> MARKQNRNSKELGLVPLTDDTSHAGPPGPGRALLECDHLRSGVPGGRRRKDWSCSLLVASLAGAFGSSFLYGYNLSVVNAPTPYIKAFYNESWERRHGRPIDPDTLTLLWSVTVSIFAIGGLVGTLIVKMIGKVLGRKHTLLANNGFAISAALLMACSLQAGAFEMLIVGRFIMGIDGGVALSVLPMYLSEISPKEIRGSLGQVTAIFICIGVFTGQLLGLPELLGKESTWPYLFGVIVVPAVVQLLSLPFLPDSPRYLLLEKHNEARAVKAFQTFLGKADVSQEVEEVLAESRVQRSIRLVSVLELLRAPYVRWQVVTVIVTMACYQLCGLNAIWFYTNSIFGKAGIPPAKIPYVTLSTGGI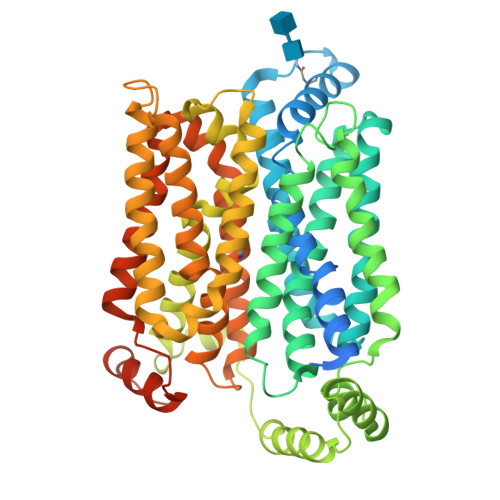ETLAAVFSGLVIEHLGRRPLLIGGFGLMGLFFGTLTITLTLQDHAPWVPYLSIVGILAIIASFCSGPGGIPFILTGEFFQQSQRPAAFIIAGTVNWLSNFAVGLLFPFIQKSLDTYCFLVFATICITGAIYLYFVLPETKNRTYAEISQAFSKRNKAYPPEEKIDSAVTDGKINGRPGTENLYFQ>MASMTGGQQMGRGSRKMATATVATTPEGIPVIILKEGSSRTYGKEALRANIAAVKAIEEALKSTYGPRGMDKMLVDSLGDITITNDGATILDKMDLQHPTGKLLVQIAKGQDEETADGTKTAVILAGELAKKAEDLLYKEIHPTIIVSGYKKAEEIALKTIQEIAQPVTINDTDVLRKVALTSLGSKAVAGAREYLADLVVKAVAQVAELRGDKWYVDLDNVQIVKKHGGSVNDTQLVYGIVVDKEVVHPGMPKRIENAKIALLDASLEVE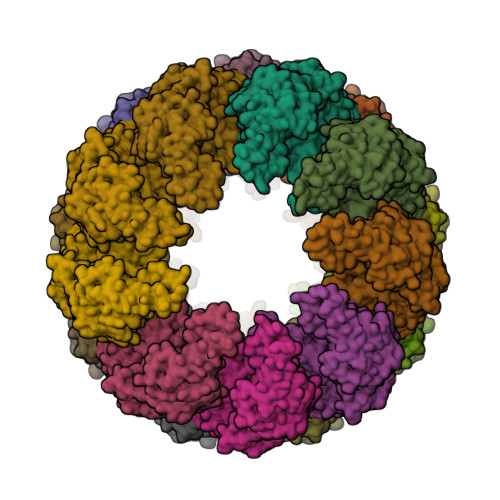KPELDAEIRINDPTQMHKFLEEEENILKEKVDKIAATGANVVICQKGIDEVAQHYLAKKGILAVRRAKKSDLEKLARATGGRVISNIDELTSQDLGYAALVEERKVGEDKMVFVEGAKNPKSVSILIRGGLERVVDETERALRDALGTVADVIRDGRAVAGGGAVEIEIAKRLRKYAPQVGGKEQLAIEAYANAIEGLIMILAENAGLDPIDKLMQLRSLHENETNKWYGLNLFTGNPEDMWKLGVIEPALVKMNAVKAATEAVTLVLRIDDIVAAGKKSGSEPSGKKEKDKEEKSSED[6x]>[2x]KHTGYVGLKNQGATCYMNSLLQTLFFTNQLRKAVYMMPTEGDDSSKSVPLALQRVFYELQHSDKPVGTKKLTKSFGWETLDSFMQHDVQELCRVLLDNVENKMKGTCVEGTIPKLFRGKMVSYI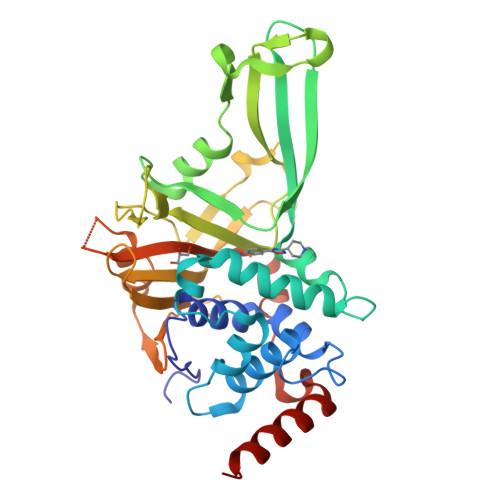QCKEVDYRSDRREDYYDIQLSIKGKKNIFESFVDYVAVEQLDGDNKYDAGEHGLQEAEKGVKFLTLPPVLHLQLMRFMYDPQTDQNIKINDRFEFPEQLPLDEFLQKTDPKDPANYILHAVLVHSGDNHGGHYVVYLNPKGDGKWCKFDDDVVSRCTKEEAIEHNYGGHDDDLSVRHCTNAYMLVYIRESKLSEVLQAVTDHDIPQQLVERLQEEKRIEAQK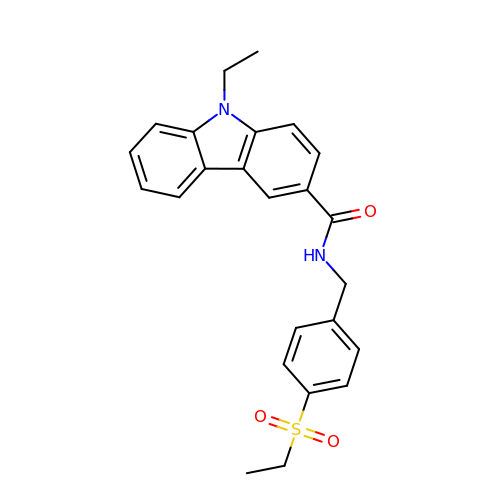9-ethyl-~{N}-[(4-ethylsulfonylphenyl)methyl]carbazole-3-carboxamide | C24 H24 N2 O3 S | KZKZVXAMNPTZPQ-UHFFFAOYSA-N>[2x]GQDKAAFEPAHLQGIWQLCHYVSENPDIPGVLKPSNTFKVLSDDGRIVNFTIRP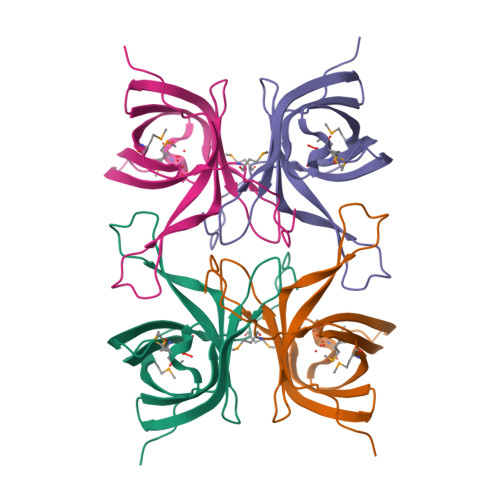GTDAIITGYGTYRQISAAAYKESIEKNIHLPMLDNKDNILEFEMGAGGVMYLKYFIEKDLNGNELNTWFHETWKRVTMPPVFPEDIVR>[2x]HHPCCSNPCQNRGECMSTGFDQYKCDCTRTGFYGENCTTPEFLTRIKLLLKPTPNTVHYILTHFKGVWNIVNNIPFLRSLIMKYVLTSR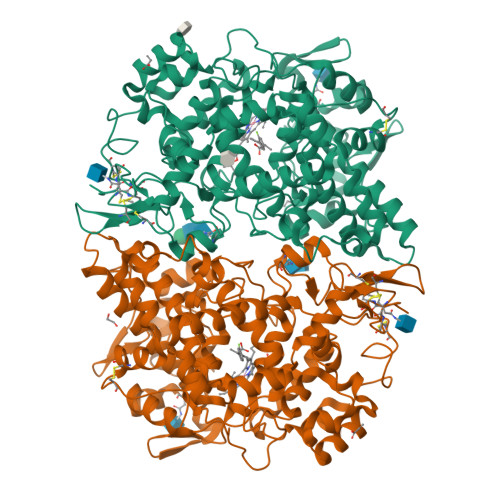PYLIDSPPTYNVHYGYKSWEAFSNLSYYTRALPPVADDCPTPMGVKGNKELPDSKEVLEKVLLRREFIPDPQGSNMMFAFFAQHFTHQFFKTDHKRGPGFTRGLGHGVDLNHIYGETLDRQHKLRLFKDGKLKYQVIGGEVYPPTVKDTQVEMIYPPHIPENLQFAVGQEVFGLVPGLMMYATIWLREHNRVCDILKQEHPEWGDEQLFQTSRLILIGETIKIVIEDYVQHLSGYHFKLKFDPELLFNQQFQYQNRIASEFNTLYHWHPLLPDTFNIEDQEYSFKQFLYNNSILLEHGLTQFVESFTRQIAGRVAGGRNVPIAVQAVAKASIDQSREMKYQSLNEYRKRFSLKPYTSFEELTGEKEMAAELKALYSDIDVMELYPALLVEKPRPDAIFGETMVELGAPFSLKGLMGNPICSPQYWKPSTFGGEVGFKIINTASIQSLICNNVKGCPFTSFNVQ> MKNKVQLITYADRLGDGTIKSMTDILRTRFDGVYDGVHILPFFTPFDGADAGFDPIDHTKVDERLGSWDDVAELSKTHNIMVDAIVNHMSWESKQFQDVLAKGEESEYYPMFLTMSSVFPNGATEEDLAGIYRPRPGLPFTHYKFAGKTRLV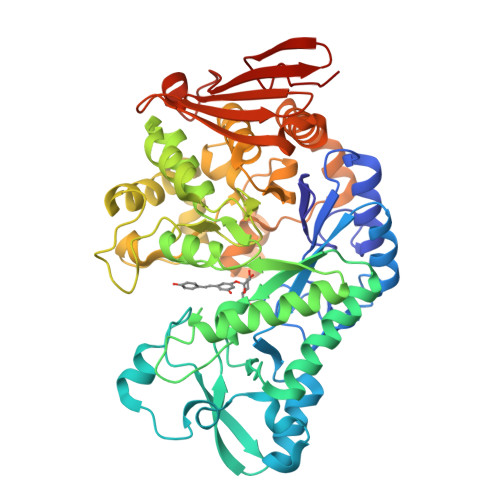WVSFTPQQVDIDTDSDKGWEYLMSIFDQMAASHVSYIRLNAVGYGAKEAGTSCFMTPKTFKLISRLREEGVKRGLEILIEVHSYYKKQVEIASKVDRVYDFALPPLLLHALSTGHVEPVAHWTDIRPNNAVTVLDTHDGIGVIDIGSDQLDRSLKGLVPDEDVDNLVNTIHANTHGESQAATGAAASNLDLYFVNSTYYSALGCNDQHYIAARAVQFFLPGVPQVYYVGALAGKNDMELLRKTNNGRDINRHYYSTAEIDENLKRPVVKALNALAKFRNELDAFDGTFSYTTDDDTSISFTWRGETSQATLTFEPKRGLGVDNTTPVAMLEWEDSAGDHRSDDLIANPPVVA>[10x]GHMNSFVGLRVVAK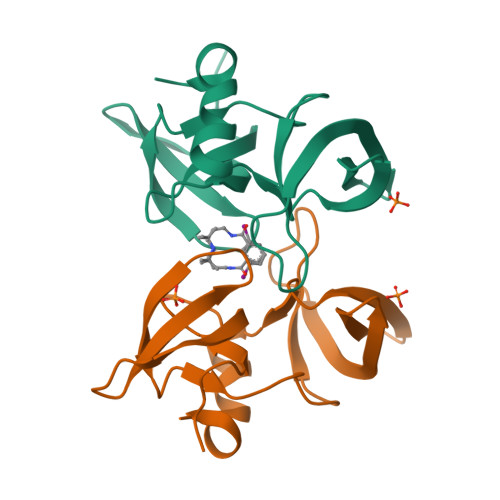WSSNGYFYSGKITRDVGAGKYKLLFDDGYECDVLGKDILLCDPIPLDTEVTALSEDEYFSAGVVKGHRKESGELYYSIEKEGQRKWYKRMAVILSLEQGNRLREQYGLG>[3x]MNHKVHHHHHHIEGAAMNEFARKKRALEHSRRINAGDLDAIIDLYAPDAVLEDPVGLPPVTGHDALRAHYEPLLAAHLREEAAEPVAGQDATHALIQISSVMDYLPVGPLYAERGWLKAPDAPGTARIHRTAMLVIRMDASGLIRHLKSYWGTSDLSGGSGPAADEAARKQMAVDYAERINAGDIEGVLDLFTDDIVFEDPVGRPPMVGKDDLRRHLELAVSCGTHEVPDPPMTSMDDRFVVTPTTVTVQRPRPMTFRIVGIVELDEHGLGRRVQAFWGVTDVTMDDRVQAFWGVTDVTMDD;> MNHKVHHHHHHIEGAAMNEFARKKRALEHSRRINAGDLDAIIDLYAPDAVLEDPVGLPPVTGHDALRAHYEPLLAAHLREEAAEPVAGQDATHALIQISSV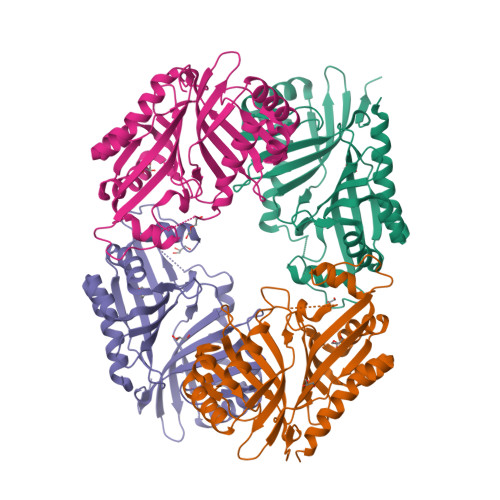MDYLPVGPLYAERGWLKAPDAPGTARIHRTAMLVIRMDASGLIRHLKSYWGTSDLSGGSGPAPDEAARKQMAVDYAERINAGDIEGVLDLFTDDIVFEDPVGRPPMVGKDDLRRHLELAVSCGTHEVPDPPMTSMDDRFVVTPTTVTVQRPRPMTFRIVGIVELDEHGLGRRVQAFWGVTDVTMDDRVQAFWGVTDVTMDD>[2x]SNAMDK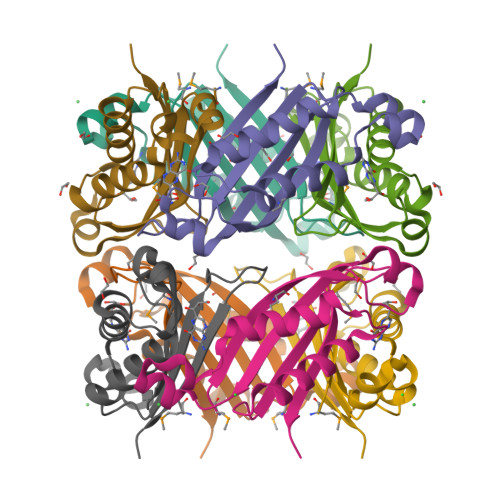IYIHDMEFYGYHGVFPEENKLGQRFKVDLTVELDLKRAGESDDLEHSVNYGELFELCRKVVEDRTYKLVESIAENIATDILKQYESISRCTIKVIKPDPPIPGHYRAVAVEITRERP>MGHQNAAVSENQNHDDGAASSPGFKLVGFSKFVRKNPKSDKFKVKRFHHIEFWCGDATNVARRFSWGLGMRFSAKSDLSTGNMVHASYLLTSGDLRFLFTAPYSPSLSAGEIKPTTTASIPSFDHGSCRSFFSSHGLGVRAVAIEVEDAESAFSISVANGAIPSSPPIVLNEAVTIAEVKLYGDVVLRYVSYKAEDTEKSEFLPGFERVEDASSFPLDYGIRRLDHAVGNVPELGPALTYVAGFTGFHQFAEFTADDVGTAESGLNSAVLASNDEMVLLPINEP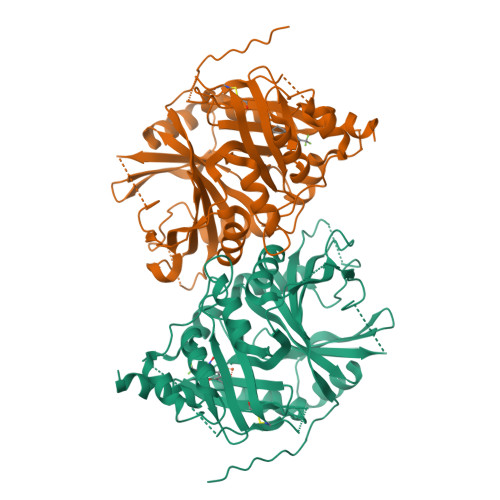VHGTKRKSQIQTYLEHNEGAGLQHLALMSEDIFRTLREMRKRSSIGGFDFMPSPPPTYYQNLKKRVGDVLSDDQIKECEELGILVDRDDQGTLLQIFTKPLGDRPTIFIEIIQRVGCMMKDEEGKAYQSGGCGGFGKGNFSELFKSIEEYEKTLEAKQLVG[4x]>MVGLIWAQATSGVIGRGGDIPWRLPEDQAHFREITMGHTIVMGRRTWDSLPAKVRPLPGRRNVVLSRQADFMASGAEVVGSLEEALTSPETWVIGGGQVYALALPYATRCEVTEVDIGLPREAGDALAPV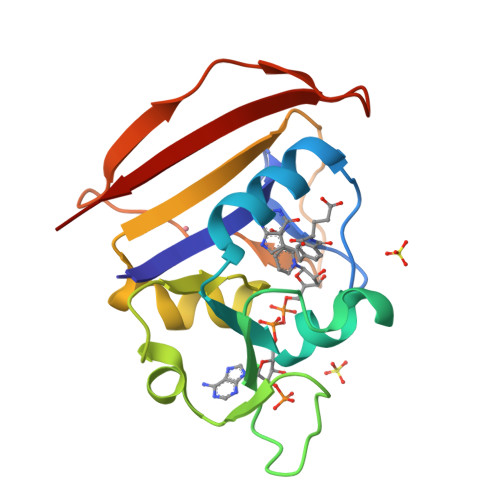LDETWRGETGEWRFSRSGLRYRLYSYHRS[2x]>WGAQGHRLVAEVADARLNPTARAEVDRLLATEPDATLASIAPWADQLRAKDPGLGRRSAGWHYVNIAEDNCHYEAPKHCRNGNCIVEALKAQSTILGDRSLTDGERLQALKFVVHLVGDIHQPMHAGYAHDKGGNDFQLQFGNRGTNLHSLWDSGMLNTRKLDDAGYLPLLQSQRAPKLARQSNPQRDPQTWAEASCRISMQAGVYPATRKIGDEYTERYRPLAEAQLRLAGENLAQLLNRVLGARLEHHHHHH[2x]

Nucleases of the S1/P1 family have important applications in biotechnology and molecular biology. We have performed structural analyses of SmNuc1 nuclease from Stenotrophomonas maltophilia, including RNA cleavage product binding and mutagenesis in a newly discovered flexible Arg74‐motif, involved in substrate binding and product release and likely contributing to the high catalytic rate. The activity of SmNuc1 towards c‐di‐GMP in crystal resulted in a distinguished complex with the emerging product 5′‐GMP. This enzyme from an opportunistic pathogen relies on specific architecture enabling high performance under broad conditions, attractive for biotechnologies.

Purine nucleotide binding differs compared to pyrimidines, confirming the plasticity of the active site.> SNASAFTEGTDYMVLEKPIPNADKTLIKVFSYACPFCYKYDKAVTGPVSDKVADLVTFTPFHLETKGEYGKQASEVFAVLIAKDKAAGISLFDAKSQFKKAKFAWYAAYHDKKERWSDGKDPAA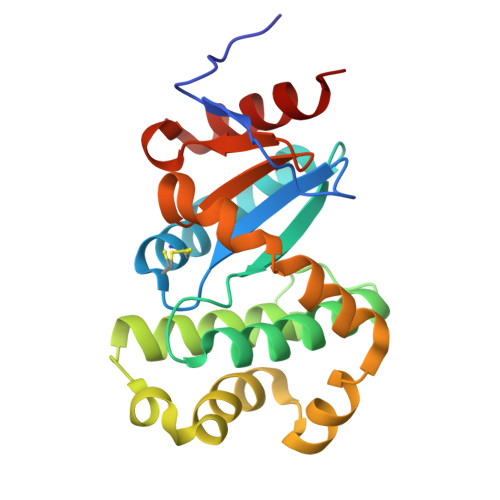FIKTGLDAAGMSQADFEAALKDPAVQETLEKWKAAYDVAKIQGVPAYVVNGKYLIYTKNIKSIDSMAELVRELATKK>[4x]MSQSNRELVVDFLSYKLSQKGYSWSQFSDVEENRTEAPEETEAERETPSAINGNPSWHLADSPAVNGATGHSSSLDAREVIPMAAVKQALREAGDEFELRYRRAFSDLTSQLHITPG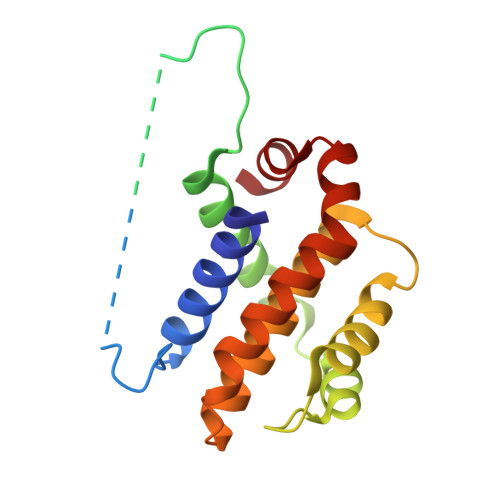TAYQSFEQVVNELFRDGVNWGAIVAFFSFGGALCVESVDKEMQVLVSRIASWMATYLNDHLEPWIQENGGWDTFVDLYG1-{5-deoxy-5-[4-(ethoxycarbonyl)piperidin-1-yl]-alpha-L-arabinofuranosyl}pyrimidine-2,4(1H,3H)-dione | C17 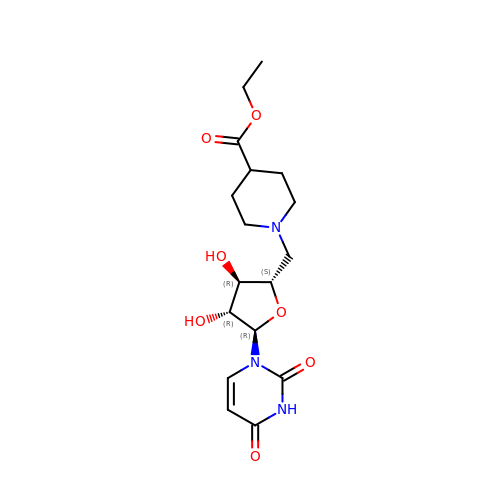H25 N3 O7 | JCIDLMJUELAXRU-SPWCGHHHSA-N1-cyclohexyl-3-[(1S,2S,3S,4R,5R)-3-hydroxy-4-(piperidin-1-yl)-6,8-dioxabicyclo[3.2.1]octan-2-yl]urea 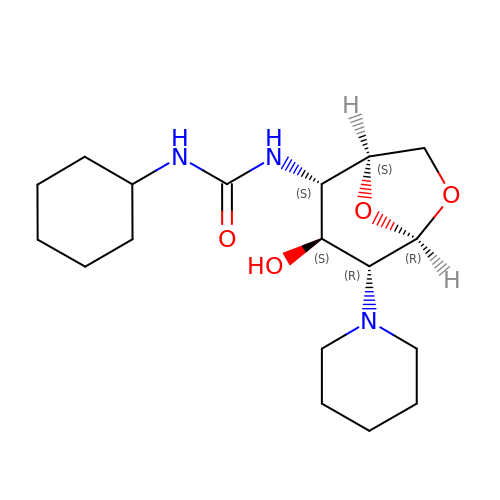| C18 H31 N3 O4 | NLUHIVDPQQPQPD-OVYGPGRDSA-N>[3x]MRIVQPVIEQLKAQSHPVCHYIYDLVGLEHHLQHITSSLPSNCQMYYAMAANSERTILDTISQYVEGFEVASQGEIAKGLAFKPANHIIFGGPGKTDEELRYAVSEGVQRIHVESMHELQRLNAILEDEDKTQHILLRVNLAGPFPNATLHMAGRPTQFGISEDEVDDVIEAALVMPNIHLDGFHFHSISNNLDSNLHVDVVKLYFKKAKSWSEKHRFPLKHINLGGGIGVNYADLTSQ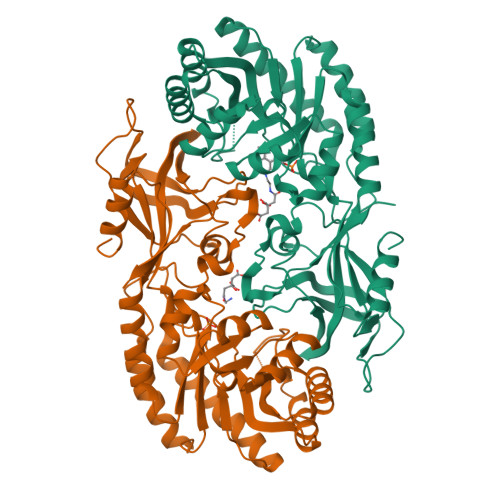FEWDNFVENFKTLIVEQEMEDVTLNFECGRFIVAHIGYYVTEVLDIKKVHGAWYAILRGGTQQFRLPVSWQHNHPFEIYRYKDNPYSFEKVSISRQDTTLVGQLCTPKDVFAREVQIDAISTGDVIVFKYAGAYGWSISHHDFLSHPHPEFIYLTQTKEDEHHHHHH>MAHHHHHHMSAPSKPSDAVARGTLYIVAAPSGAGKSSIVNATLARDPQIALSISFTSRAMRPGEVNGQHYHFVSAEKFEQMIAAGDFFEHAWVHGDWKGTARQSVEPQLAAGQDVLLEIDWQGAQQVRQLVPGTVTVFILPPSKQALQDRMRKRGQDSEAVIAQRLGAARDEMLHFNEFDYVIVNEVFDTAVDELCAIFT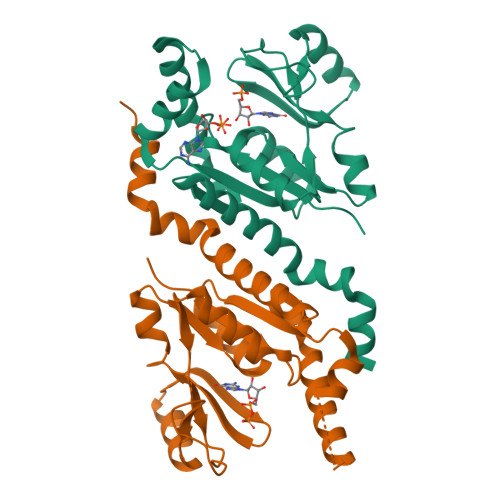ASRLRREAQKVRHAGLIQALLTPDPGATD[8x]>[2x]MNHKVHHHHHHIEGRHMPAPAGDAAGLGLEATEHPLLATATELPDGGYLFTGRLALREHPWLADHTIAGTTIVPGTAFVELALHAADIAGCDEITELVLHTPLVLSTQSSSLLQVAVGPADPSGARSLTIRSHGEDVRLWVEHADGSIGPGETAPELPEPVRVGLVPRGSGMTGSEEAFASADGTD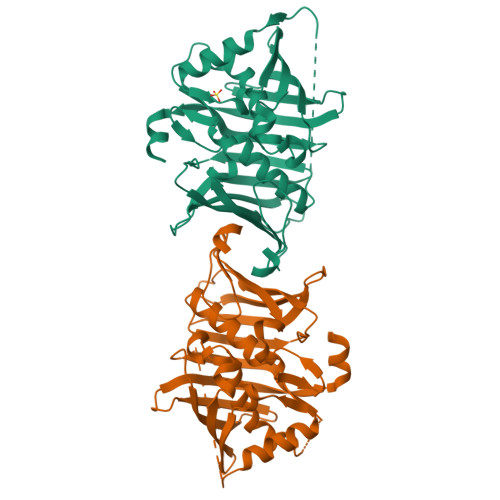EAWPPPGGDAWDTAGLYARLADRGFQYGETFRGLRAAWSSGEDIYADVEVGAPASSPKPEAFHVHPALLDAALHAALGPLLDGEEGLFLPFALRRVRVHHSGAKSLRVHITPDGDKSVSLSAVDAAGNAVVSVGSVALRPVSSAQLAAAAGRNG3-(6-methoxynaphthalen-2-yl)-1-(propan-2-yl)-1H-pyrazolo[3,4-d]pyrimidin-4-amine 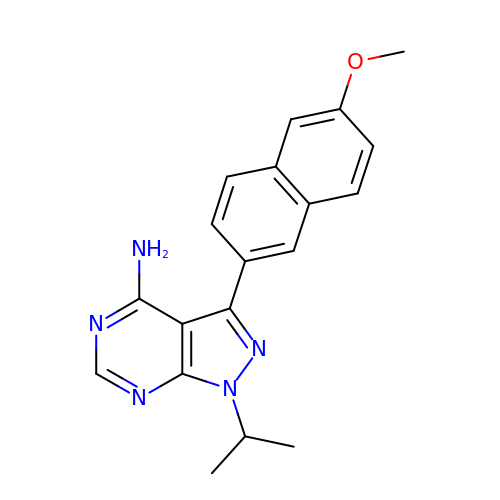| C19 H19 N5 O | YTSDNPLOCDVGNB-UHFFFAOYSA-N> RDQEQYIHRKCYQEFAHCYLVKYKTPQPWPNEGLIADQCPLPGLADVSFYPYQAIWDYYAKIENIRPANWTSSKLYGKARMGSYYIPKRLRNINNTHILFCSDVLYSKWYNLQN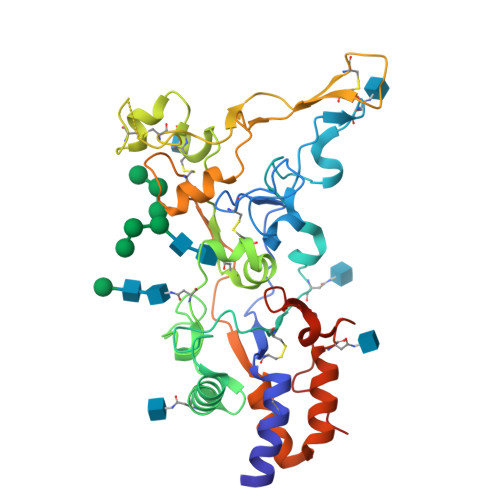SILQNENELTKRLSNLTIGNKLKNRALPYEWAKGGLNRLFRNISVLDVCSRPEMVLLLNKTYYTFSLWEGDCNITRYNVNETVPECKDFPHRRFNDHPYSCRLWRYREGKEEVKCLTSDHTRCLYYPEYSNPEALFDFGFLSYMRNFPGPQCIESTSIRQQDYEVYSIYQECKLASKTYGIDSVLFSLKNFLNYTGKPVNEMPNARAFVGLIDPKFPPTYPDDDDK>[2x]MQEEPTNIPRPDNAELLVASEVAIENAAIALSEIVSVVNTSDGRIEVFGVGTDNAVWHNRQTAPHSGSSWTGWISLNGKVTSKPVVYINTDGRLEVFARGTDNALWHIWQTATNAGWSNWQSLGGTITSNPAVYVNTDGRIDVFARGTDNALWHISQTAAHSGPWSSWQSLNGVITSNPAVHINSDGRLEVFARGTDNALW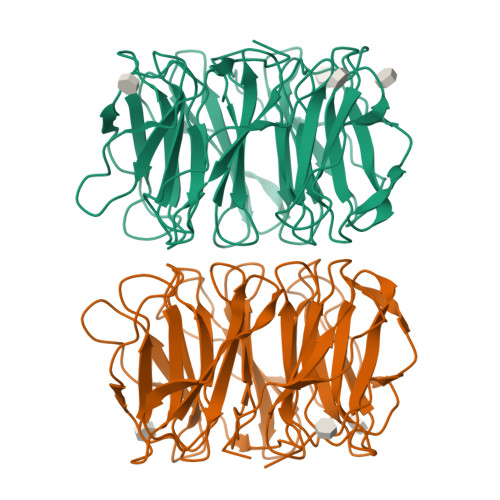HIWQTAPDSNQWSGWDSLGGVITSDPVVIGTADGRLEVFARGSNNALYHIWQTVPHGGPWSNWASLNGVITSAPAVVKNSDGRLEVFARGTNNALYHIWQTVSHSGPWSNWATLNGTITSAPTAVEDADGRLEVFARGTDNALWNIWQATPSWSAWVSLKGSLIDASAIK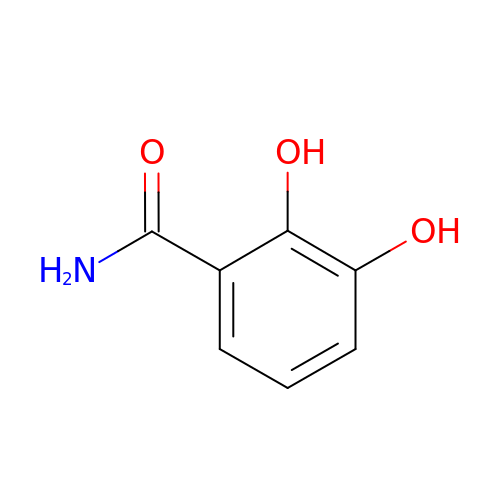2,3-DIHYDROXYBENZAMIDE | C7 H7 N O3 | QCIDBNKTKNBPKM-UHFFFAOYSA-N Keap1 (Kelch-like ECH-associated protein 1) is a multi-domain protein which plays a key role in the regulation of Nrf2, a transcription factor that mediates the expression of a large array of cytoprotective enzymes in response to electrophilic and oxidative assault. In common with related family members, it acts in concert with members of the CRL3 class of Cullin-RING-Ligase E3 ligases to provide substrate-specific recruitment for ubiquitination, and consists of a three domain architecture composed of an N-terminal BTB (Broad complex, Tramtrack, and Bric-a-Brac) domain, an intervening region (IVR) or BACK domain, and a C-terminal Kelch repeat domain. Keap1 is known to dimerize through its BTB domain, and models of the mechanism of action require dimerization for constructive engagement with the Nrf2 substrate. In the case of Keap1, the BTB domain is unique in providing an additional role in the sensing of oxidative stress.

In addition, we also report here the structure of a mutant form of the Keap1 BTB domain where the reactive cysteine at position 151 has been mutated to tryptophan. This mutation has been shown to constitutively activate the Nrf2 pathway through antagonism of Keap1, and we discuss this structure in the context of both apo and CDDO-bound forms of the protein. In order to gain further insight into mechanism of action of modifications to Cys 151, we also solved the structure of the Keap1 BTB domain C151W mutant. In addition, we have recently demonstrated that introduction of the C151W mutation disrupts the interaction of Cul3 with full-length Keap1 using a TR-FRET assay (manuscript in preparation). An overlay with the apo C151 structure reveals a change in rotamer for the side-chain of Arg 135, but no significant conformational movements with the potential to disrupt the binding with Cul3. In addition, the structure of the C151W mutant presented here shows no evidence for disruption of the BTB homodimerization interface. Superposition of the C151W and CDDO-bound structures shows that the side-chain of Trp 151 adopts a rotamer in which the indole ring is orthogonal to the CDDO ring system, although occupying a similar region of space to the lower portion of the antagonist. Neither the binding of CDDO, nor the C151W mutation appears to lead to large conformational changes, and although we cannot preclude the possibility that additional effects are relevant in solution, or in full-length Keap1, the structures presented here suggest a model where dissociation of Cul3 may be driven by direct steric hindrance with residues in its N-terminal tail.

> GSHMGNRTFSYTLEDHTKQAFGIMNELRLSQQLCDVTLQVKYQDAPAAQFMAHKVVLASSSPVFKAMFTNGLREQGMEVVSIEGIHPKVMERLIEFAYTASISMGEKWVLHVMNGAVMYQIDSVVRACADFLVQQLD>SMIFKPEELRQALMPTLEALYRQDPESLPFRQPVDPQLLGIPDYFDIVKSPMDLSTIKRKLDTGQYQEPWQYV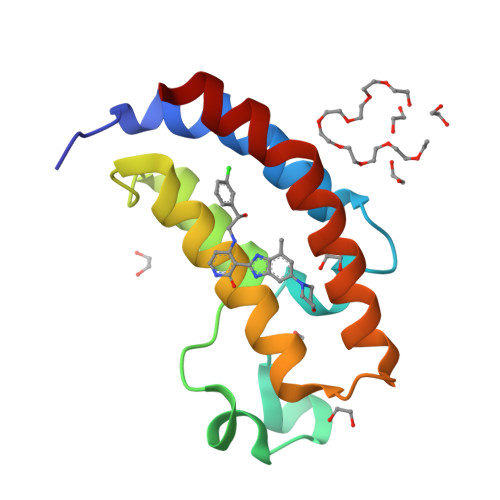DDIWLMFNNAWLYNRKTSRVYKYCSKLSEVFEQEIDPVMQSLG[2x]> GPGAPNVLNWEQVQRLDGILSETIPIHGRGNFPTLELQPSLIVKVVRRRLAEKRIGVRDVRLNGSAASHVLHQDSGLGYKDLDLIFCADLRGEGEFQTVKDVVLDCLLDFLPEGVNKEKITPLTLKEAYVQKMVKVCNDSDRWSLISLSNNSGKNVELKFVDSLRRQFEFSVDSFQIKLDSLLLFYECSENPMTETFHPTIIGESVYGDFQEAFDHLCNKIIATRNPEEIRGGGLLKYCNLLVRGFRPASDEIKTLQRYMCSRFFIDFSDIGEQQRKLESYLQNHFVGLEDRKYEYLMTLHGVVNESTVCLMGHERRQTLNLITMLAIRVLADQNV;> GPGAPDEVIDEEVNIEFEAYSLSDNDYDGIKKLLQQLFLKAPVNTAELTDLLIQQNHIGSVIKQTDVEVFGFISLLNLTERKGTQCVEQIQELVLRFCEKNCEKSMVEQLDKFLNDTTKPVGLLLSERFINVPPQIALPMYQQLQKELAGAHRTNKPCGKCYFYLLISKTFVEAGQHNGGSRGQVTALVSLKAGLIQSRSTLSDFQGTFMTVGIALS

The FAM46 (also known as TENT5) proteins are noncanonical poly(A) polymerases (PAPs) implicated in regulating RNA stability. Here, we report that the nuclear protein BCCIPα, but not the alternatively spliced isoform BCCIPβ, binds FAM46 and inhibits their PAP activity. Unexpectedly, our structures of the FAM46A/BCCIPα and FAM46C/BCCIPα complexes show that, despite sharing most of the sequence and differing only at the C-terminal portion, BCCIPα adopts a unique structure completely different from BCCIPβ. A helix-loop-helix segment in BCCIPα inserts into the active site cleft of FAM46, thereby inhibiting the PAP activity.

The FAM46A/BCCIPα-ΔL complex yielded better crystals. The following description of the FAM46A/BCCIPα structure will refer to this higher-resolution structure. BCCIPα forms a large binding interface with the active site cleft of FAM46A, burying ~2600-Å2 solvent-accessible area. The strand at the outer edge of the active site cleft of FAM46A (residues 189 to 196) packs against strand β1 in BCCIPα in an antiparallel fashion, integrating the β sheets in the two proteins into one extended β sheet. Strand β1 in BCCIPα and the edge β strand in FAM46A form seven backbone hydrogen bonds to join the β sheets in the two proteins together. However, CPB1 of Plk4 leaves the active site in FAM46C unoccupied, and its binding does not affect the PAP activity of FAM46 (5). In contrast, as shown in Fig. 3A, helices B and C and the loop between them at the bottom of the β sheet in BCCIPα are wedged into the active site cleft in FAM46A. Lys155 at the tip of the loop between helices B and C in BCCIPα sticks deep into the active site and makes a direct interaction with the catalytic residues Asp141 and Glu215. To accommodate BCCIPα, the C-terminal lobe of FAM46 rotates away substantially from the N-terminal lobe and creates a larger opening, as shown by a comparison of the complex structure with FAM46C in the apo-state. Most of the residues in FAM46A involved in the binding interface are conserved in other FAM46 family members, which underlies the interaction of BCCIPα with all the FAM46 proteins.> MSIKDSIGLRIKTERECQQMSREVLCLDGAELTVRQLIRIEKGESLPSLDKLSYIAKRLGKSMADLLDHDRIEIPDTYYEMKNRLIKFPTYGDKERVKQKLDLIEDVYNQFFDILPEEELLTLD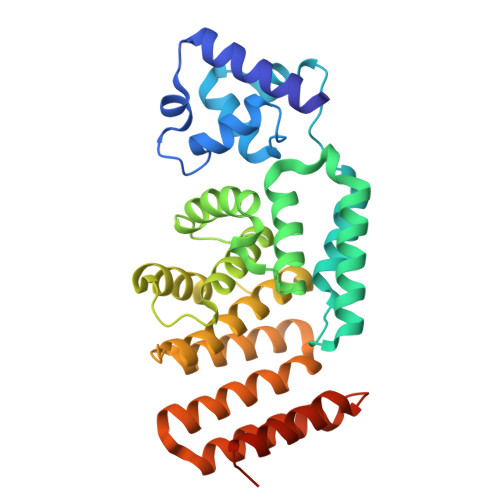ILENILSFTSWEERPKVEEIYEDLFEQVKRKKKFSTNDLLVIDYYFYHLYGRKQYDKKIFDRIVDRVLKQNIPTDDAYNIALFNDLMAIAGLKISLESFKDFLTVIDKLLAVIEKSQFHSYKPGVYILEAKYELIHNGNKKKATENYDKAIMFASVLEDSVLEEKTRAEKAADGLGAGWSHPQFEK> ATATAATPAAEATSRGWNDYSCKPSAAHPRPVVLVHGTFGNSIDNWLVLAPYLVNRGYCVFSLDYGQLPGVPFFHGLGPIDKSAEQLDVFVDKVLDATGAPKADLVGHSQGGMMPNYYLKFLGGADKVNALVGIAPDNHGTTLLGLTKLLPFFPGVEKFISDNTPGLADQ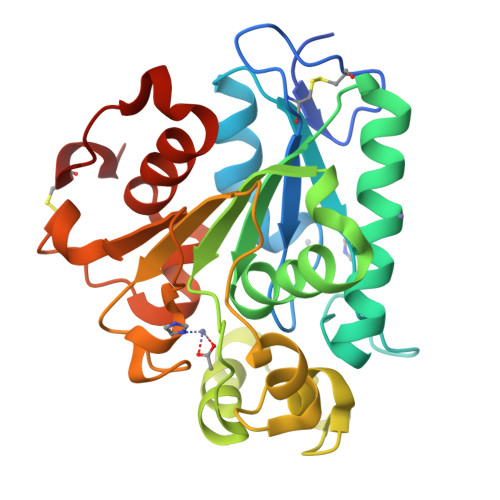VAGSPFITKLTAGGDTVPGVRYTVIATKYDQVVTPYRTQYLDGPNVRNVLLQDLCPVDLSEHVAIGTIDRIAFHEVANALDPARATPTTCASVIG> TRGFRWDLCQRGRRRWVHINYPPRNRSTVQMLDESHEKLVFVCNGYIDRLDPRLLPERLRKRLERNRKAALTRF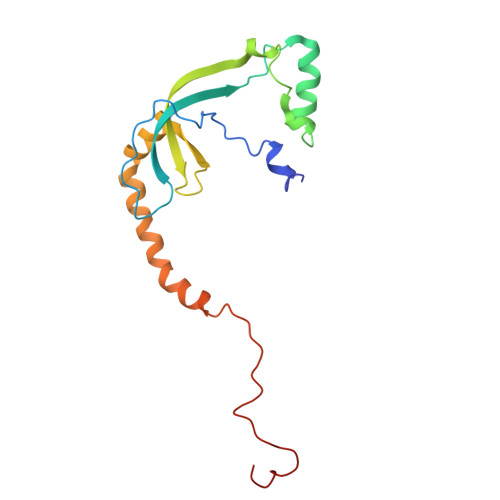DGKLPWGQAVESAIKRIHTPCLAFAQAHSHHLLEAFSMAEVLEIEKLIPEIREAFKASKAKLAEQEAQDKFTRHVSVDLVDLKEDPVSFPFTLK Arachinoyl-CoA 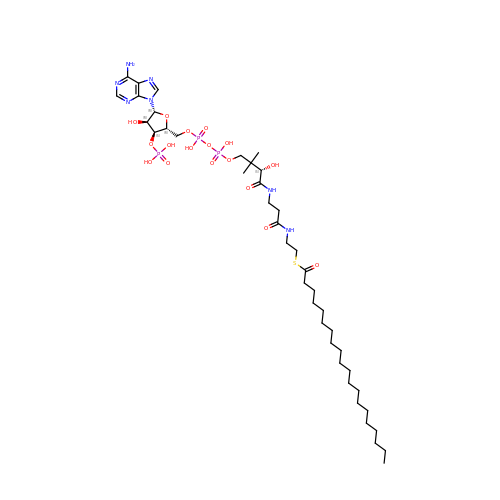| C41 H74 N7 O17 P3 S | JYLSVNBJLYCSSW-DLATUHJOSA-N> APKVVKFSYMWTINNFSFCREEMGEVIKSSTFSSGANDK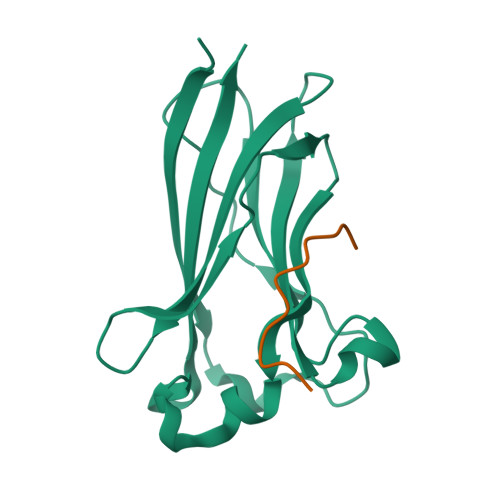LKWCLRVNPKGLDEESKDYLSLYLLLVSCPKSEVRAKFKFSILNAKGEETKAMESQRAYRFVQGKDWGFKKFIRRDFLLDEANGLLPDDKLTLFCEVSVVQD;> KPLQVAAVDSSVPRTAELAG>[4x]GPVCAEASDVYSPCMIASTPPAPFSDVTAVTFDLINGKITPVGDDNWNTHIYNPPIMNVLRTAAWKSGTIHVQLNVRGAGVKRADWDGQVFVYLRQSMNPESYDARTFVISQPGSAMLNFSFDIIGPNSGFEFAESPWANQTTWYLECVATNPRQIQQFEVNMRFDPNFRVAGNILMPPFPLSTETPPL;>[4x]MEQNLFALSLDDTSSVRGSLLDTKFAQTRVLLSKAMAGGDVLLDEYLYDVVNGQDFRATVAFLRTHV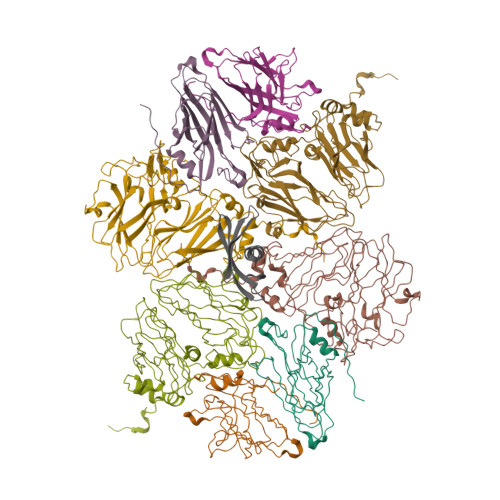ITGKIKVTATTNISDNSGCCLMLAINSGVRGKYSTDVYTICSQDSMTWNPGCKKNFSFTFNPNPCGDSWSAEMISRSRVRMTVICVSGWTLSPTTDVIAKLDWSIVNEKCEPTIYHLADCQNWLPLNRWMGKLTFPQGVTSEVRRMPLSIGGGAGATQAFLANMPNSWISMWRYFRGELHFEVTKMSSPYIKATVTFLIAFGNLSDAFGFYESFPHRIVQFAEVEEKCTLVFSQQEFVTAWSTQVNPRTTLEADGCPYLYAIIHDSTTGTISGDFNLGVKLVGIKDFCGIGSNPGIDGSRLL;> ENSLEIEELARFAVDEHNKKENALLEFVRVVKAKEQVVAGTMYYLTLEAKDGGKKKLYEAKVWVKPWENFKELQEFKPV(S)-2-methyldecanoyl-CoA | C32 H56 N7 O17 P3 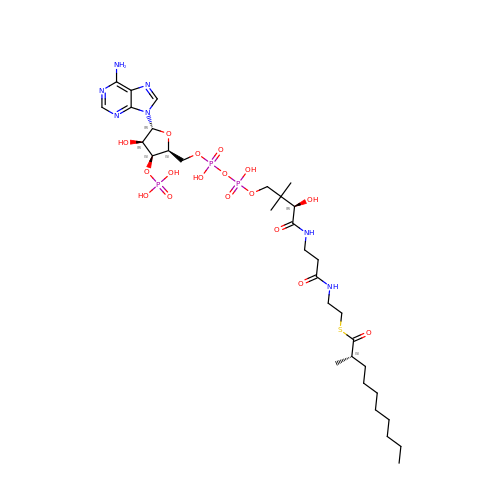S | IERLRQNOXCBECM-ZWASGNAISA-N> MNAVLSVQGASAPVKKKSFFSKFTRLNMLRLARAVIPAAVLMMFFPQLAMAAGSSGQDLMASGNTTVKATFGKDSSVVKWVVLAEVLVGAVMYMMTKNVKFLAGFAIISVFIAVGMAVVGL

DNA transfer is facilitated by a type IV secretion system (T4SS) nanomachine, embedded in the bacterial cell wall, which is extended by a long hollow filament, known as the conjugation, mating, or sex pilus. Functionally, the pilus is involved in mating pair formation (MPF), linking donors and recipients at a distance. Structures of mating or conjugation pili from the IncF and IncW incompatibility plasmids have revealed that the pilins polymerize into a helical arrangement with tightly bound phospholipid molecules, forming thin, tubular filaments ~8 nanometers in diameter that can extend several micrometers in length. Conjugation pilins are composed of three α helices, α1-3.

In IncF plasmids, MPF has been shown to enable low efficiency DNA transfer via the hollow conjugation pilus. While the IncH and IncF plasmid encode an MPFF conjugation machinery type, only the H-pilin is cyclic.>[8x]SNAPVEGSEEDKSQTGVNRASKGGLIYGNYLHLEKVLNAQELQSETKGNKIHDEHLFIITHQAYELWFKQILWELDSVREIFQNGHVRDERNMLKVVSRMHRVSVILKLLVQQFSILETMTALDFNDFREYLSPASGFQSLQFRLLENKIGVLQNMRVPYNRRHYRDNFKGEENELLLKSEQEKT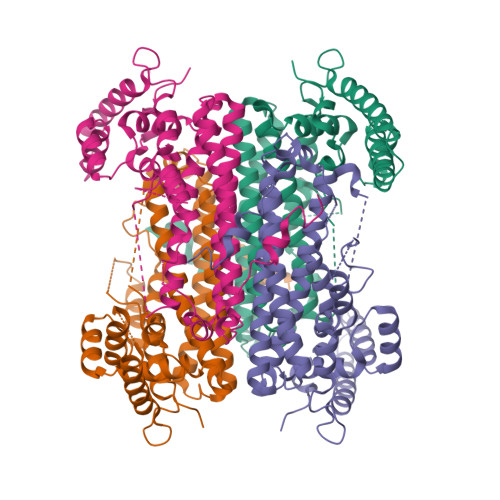LLELVEAWLERTPGLEPHGFNFWGKLEKNITRGLEEEFIRIQAKEESEEKEEQVAEFQKQKEVLLSLFDEKRHEHLLSKGERRLSYRALQGALMIYFYREEPRFQVPFQLLTSLMDIDSLMTKWRYNHVCMVHRMLGSKAGTGGSSGYHYLRSTVSDRYKVFVDLFNLSTYLIPRHWIPKMNPTIHKF> PLPEVQCFVFNVEYMNCTWQSSSEPQPTNLTLHYWYKNSDNDKVQKCSHYLFSEEITSGCQLQKKEIHLYQTFVVQLQDPREPRRQATQMLKLQNLVIPWAPENLTLHKLSESQLELNWNNRFLNHCLEHLVQYRTDWDH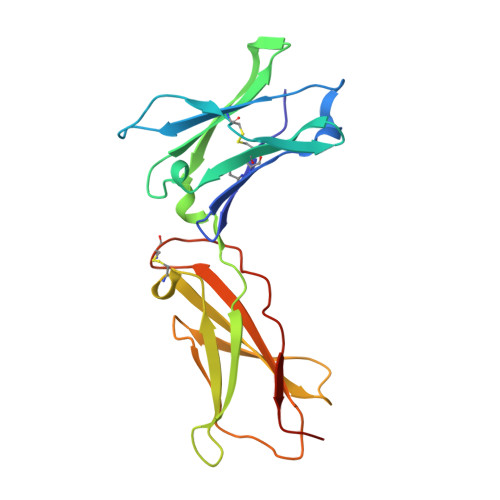SWTEQSVDYRHKFSLPSVDGQKRYTFRVRSRFNPLCGSAQHWSEWSHPIHWGSNTSKEN> GAMGSWNPKYDTRTLWTTPDTSPNCTIAQDKDSKLTLVLTKCGSQILANVSLIVVAGKYHIINNKTNPKIKSFTIKLLFNKNGVLLDNSNLGKAYWNFRSGNSNVSTAYEKAIGFMPNLVAYPKPSNSKKYARDIVYGTIYLGGKPDQPAVI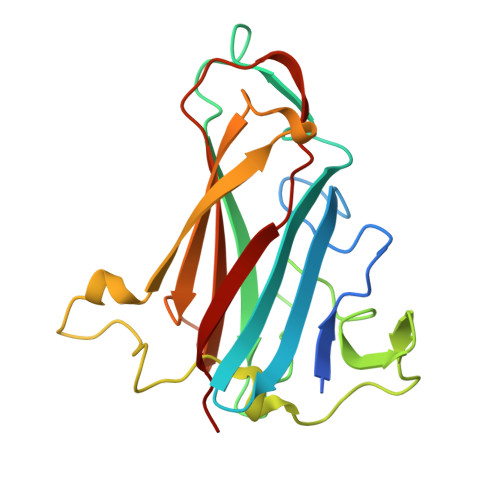KTTFNQETGCEYSITFNFSWSKTYENVEFETTSFTFSYIAQE> MTSTKKRKLEGSASESGNNTPILSAFAARQQLWAQSLVVQAQKQPQSVDNSKHVTERRSATPISAAQVLRKSKRKSPEDSPITPATPATPVETEEEKPSKPSSPRELLRHHSSFQPNNSNFQRKAGGRLVLSTPDVERFVILGNYGVKVHQGEVTIAGATLTPIDDVQWVHAPHCHALPVLRTANDTVIELLPCPTAQGLRELARLNPLFGRLW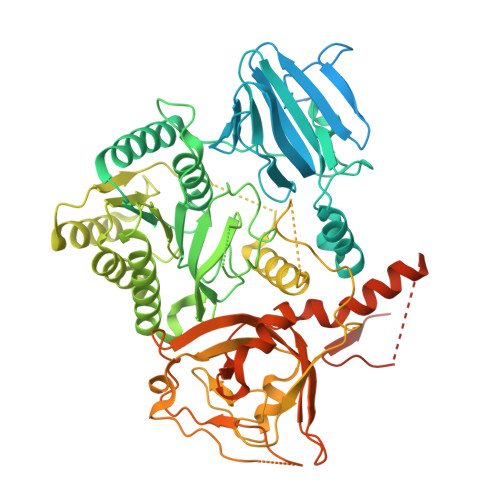NETSDTFQIIYTSADAPKRTSLRELASHPAWNKKISELLTSTRRKPSPILFICGPKSSGKSTFGRLLTNRLMTDRAGHKSRSWKPVMVLDLDPGQPEFSPPGVVSLTKLRRPNLAPPFCHPGLSFGEKGLDGGNEGMTTVRMHAIASVTPALDPAHFIACARDLFAYYRRSASQENIPLVVNTPGWIQGTGLDLLAELIAVLRPTEVLYMSEDGPEETVSALREACASSSTIPFTMLPSQPNSSGEGGGGGAASWTPATLRSMAMQSYFHLSPFSRDQQGGPGCEWNPTPLTHLCPWRVRLAGRPDERGVLGIVCYDHQYAPELVSDAINGMVMGLVRIEKKEALRGLAVPGDTSLSFTSSTSQGGCDDELDSDSNSSSAPSFTSSSPSHLNSTPLLPLIPNPTGSPLSPQYTSLVGLVLIRGVSLTASNPELHLLTPVPPSVLHSFRGDELVLVAGKFDAPTWAYVEGLYWKSNSKAAKRVDEEREDEDREESGGVEEEEEQDEVPWVEMLHGSAGRDVGSRVWRVRRDLGRS> MSQSNRELVVDFLSYKLSQKGYSWSQFSDVEENRTEAPEETEAERETPSAINGNPSWHLADSPAVNGATGHSSSLDAREVIPMAAVKQALREAGDEFELRYRRAFSDLTSQLHITPG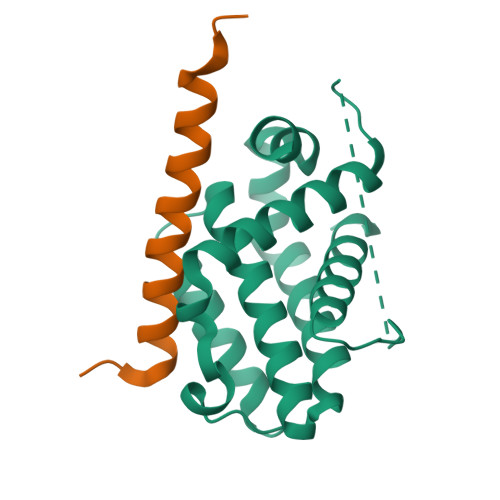TAYQSFEQVVNELFRDGVNWGRIVAFFSFGGALCVESVDKEMQVLVSRIASWMATYLNDHLEPWIQENGGWDTFVDLYG;> DLRPEIRIAQELRRIGDEFNETYTRRVFANDYR> PKHGKRYRALLEKVDPNKIYTIDEAAHLVKELATAKFDETVEVHAKLGIDPRRSDQNVRGTVSLPHGLGKQVRVLAI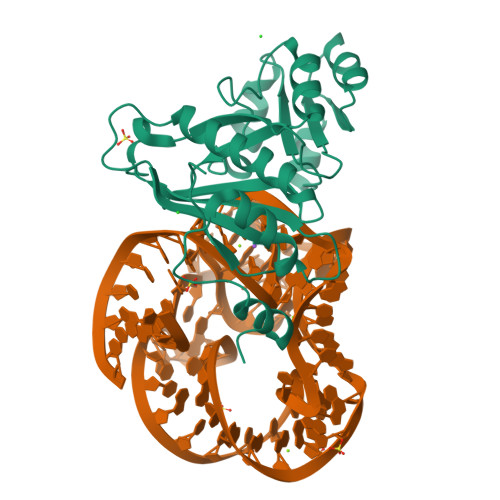AKGEKIKEAEEAGADYVGGEEIIQKILDGWMDFDAVVATPDVMGAVGSKLGRILGPRGLLPNPKAGTVGFNIGEIIREIKAGRIEFRNDKTGAIHAPVGKASFPPEKLADNIRAFIRALEAHKPEGAKGTFLRSVYVTTAMGPSVRINPHS>ASHMFRKLAAESFGTFWLVFGGSGSAVLAAGFPELGIGFAGVALAFGLTVLTMAFAVGHISGGHFNPAVTIGLWAGGRFPAKEVVGYVIAQVVGGIVAAALLYLIASGKTGFDAAASGFASNGYGEHS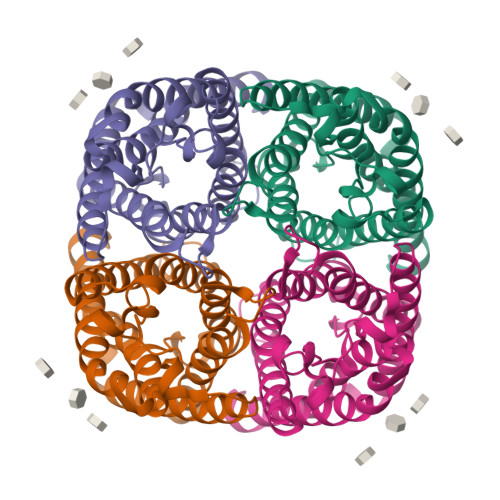PGGYSMLSALVVELVLSAGFLLVIHGATDKFAPAGFAPIAIGLALTLIHLISIPVTNCSVNPARSTAVAIFQGGWALEQLWFFWVVPIVGGIIGGLIYRTLLEKRD[2x]>[2x]MSLSLLITSITINTSHLQGMLGFYRIIGFQFTASKVDKGSEVHRAVHNGVEFSLYSIQNPQRSQIPSLQLGFQITDLEKTVQELVKIPGAMCILDPTDMPDGKKAIVL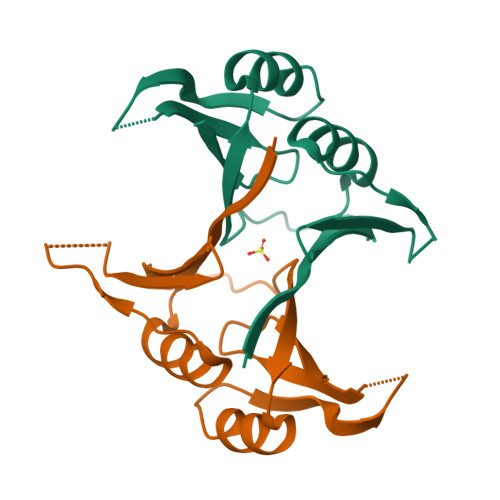DPDGHSIELCELEGHHHHHH> AEMGAAACTLLWGVSSSEEVVK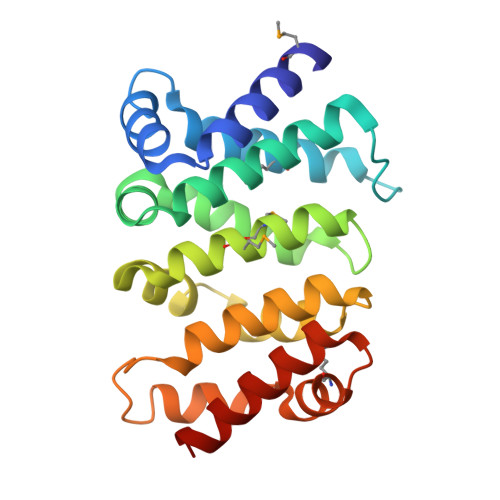AILGGDKALKFFSITGQTMESFVKSLDGDVQELDSDESQFVFALAGIVTNVAAIACGREFLVNSSRVLLDTILQLLGDLKPGQCTKLKVLMLMSLYNVSINLKGLKYISESPGFIPLLWWLLSDPDAEVCLHVLRLVQSVVLEPEVFSKSASEFRSSLPLQRILAMSKSRNPRLQTAAQELLEDLRTLEHNV>SMSKNNIFNKYPTIIHGEARGENDEFVVHTRYPRFLARKSFDDNFTGEMPAKPVNGELGQIGEPRRLAYDSRLGLWLSDFIMLDNNKPKNMEDWLGQLKAACDRIAADDLMLNEDAADLEGWDD[2x];> SMAAFKPNSINYILGLDIGIASVGWAMVEIDEE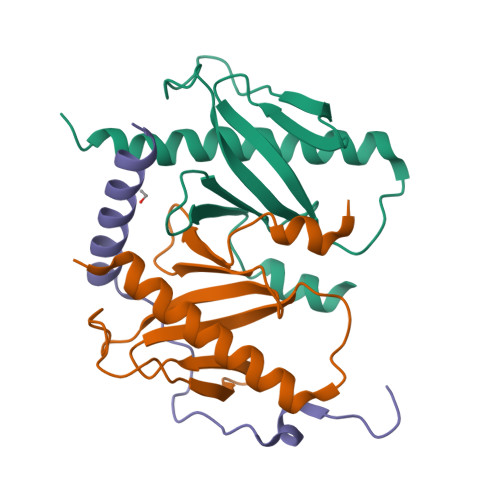ENPIRLIDLGVRVFERAEVPKTGDSLAMARRLARSVRRLTRRRAH>GAMKVEVITGEEAESNVLQMQCKLFVFDKTSQSWVAVGRGLLRLNDMASTDDGTLQSRLVMRTQGSLRLILNTKLWAQMQIDKASEKSIRITAMDTEDQGVKVFLISASSKDTGQLYAALHHRILALRSRVEQEQEAK[2x]

RanBP3 is a Ran-interacting protein with diverse roles in nuclear transport. Specifically, RanBP3 enhances the rate of NES export by increasing the affinity of CRM1 for RanGTP, thereby stabilizing the ternary CRM1/Ran/cargo complex in the nucleus. RanBP3 belongs to a class of Ran-binding proteins characterized by one or more Ran-binding domains (RBDs) of approximately 120 residues. As expected, the RanBP3 RBD adopts a pleckstrin homology fold, composed of 7 anti-parallel β-strands and a C-terminal α-helix.

We therefore pursued the structure of the RBD in its unbound form. We solved the structure at 1.61 Å resolution using experimental phases obtained from a platinum derivative, and at 2.1 Å in a second crystal form by molecular replacement. Crystal forms 1 and 2 contain two and four molecules per asymmetric unit, respectively, and aligning these structures reveals variations in the N- and C-terminal residues and in several loops, reflecting the inherent flexibility of these regions. In contrast, the β5β6 loop, whose functional role is evoked below, is highly uniform in structure, suggesting a comparatively rigid element. The strands define a continuous sheet with simple up-down topology, forming an imperfect β barrel that juxtaposes strands 4 and 6 and extrudes strand 5. The C-terminal helix caps the barrel, packing against strands 1, 2, 5 and 6.> GFPTELKPGTNQFLTTDDGVSAPILPNFHPTPCIHIPGEVRNLLELCQVETILEVNNVPTNATSLMERLRFPVSAQAGKGELCAVFRADPGRSGPWQSTLLGQLCGYYTQWSGSLEVTFMFTGSFMATGKMLIAYTPPGGPLPKDRATAMLGTHVIWD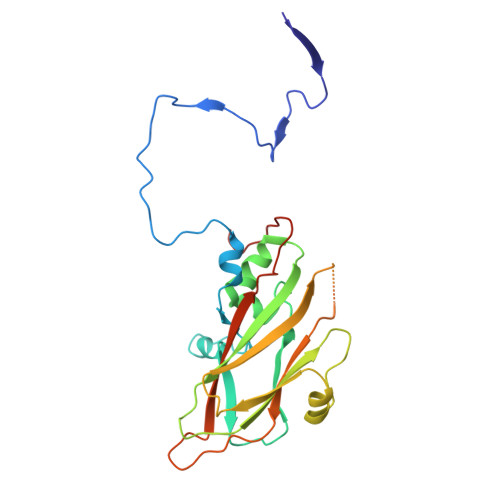FGLQSSVTLVIPWISNTHYRAHARDGVFDYYTTGLVSIWYQTNYVVPIGAPNTAYIIALAAAQKNFTMQLCKDASDILQTGTIQ>MAETKVAPN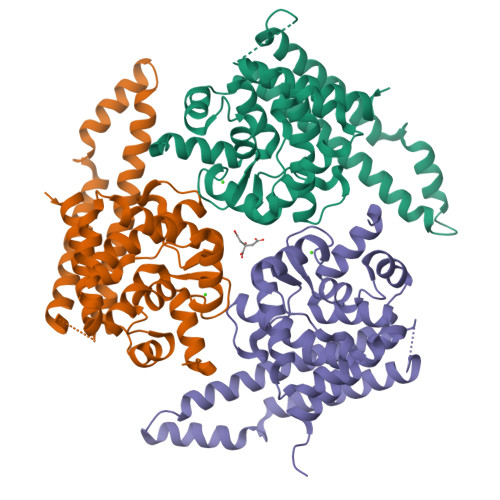LTGIEQTKAGQSFTEKLSAEAMEFFCNVAKLPFSQQAVHFLNAYWAEVSKEAEFIYSVGWETIKYADMHCKGIQLVFKYDEGNDLDFDIALYFYEQLCKFCEDPKNKNYATTYPISQPQMLTALKRKQELREKVDVNFDGRVSFLEYLLYQYKDFANPADFCTRSMNHDEHPEIKKARLALEEVNKRIRAYEEEKARLTEESKIPGVKGLGATNMLAQIDSGPLKEQLNFALISAEAAVRTASKKYGGAAYSGGAGDAGAGSSAGAIWWMNRDLEEKKKRYGPQKK[3x]>GKKEESEVLNVTESLQKESEITSFSEEEEAVLYMLSALKKNDLDMALRGCAIDETALQINFVKTAEELPGMQLIDLPAPTSDYSYYFPLTSAEMTKAYIEQFEELSTEIPEIETLEVLEIAEKKEKEREEQLAECLAAQEVSELEIYVKCGEQSYRLGFTAVQYEKNWKIHSLKEGLLYETDIPACVQMEEMREAKKTYVLPNQLTGANYFQAMPISEKTPQRAVEQFIYAIEKGDLTRALAFATTESSQDTSPELLKKQGEYAKELKTMLYGFLGTEDARLYGKSEEQLNKLRGKLNPEYMVYLDLIKVIPIETEENTETVKQYAGLYSYNGKNYLTGYTLCRQEDGWQIQ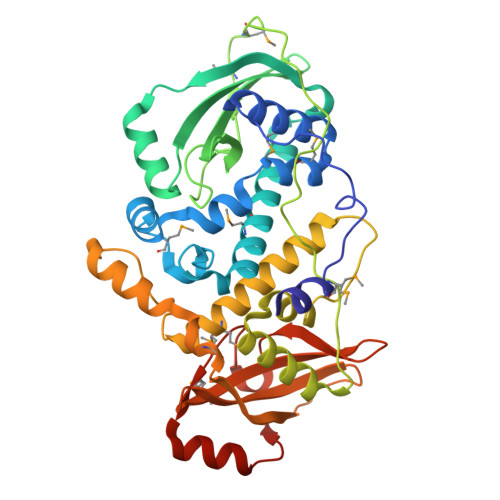SLSAPALSLESGEVMRLSKEESRKTSEQSVLKAEKNER[2x]>[2x]MGSSHHHHHHSQDPGDENLYFQSMSDADRIAALLKDRAADPVTKFSPSPYETGQFLRISERADVGTPQIDYLLATQRPDGLWGSVGFELVPTLGAVAGLSSRPEYADRAGVTDAVARACEKLWELALGEGGLPRLPDTVASEIIVPSLIDLLGEVLQRHRPAAGGKAGHEQEFPSPPGAKPELWRRLSDRIARGQAIPETAWHTLEAFHPLPEQFAATVTPAADGAVTCSPSSTAAWVSAVGTDAGASTRAYLDEAQSRYGGAIPMGSS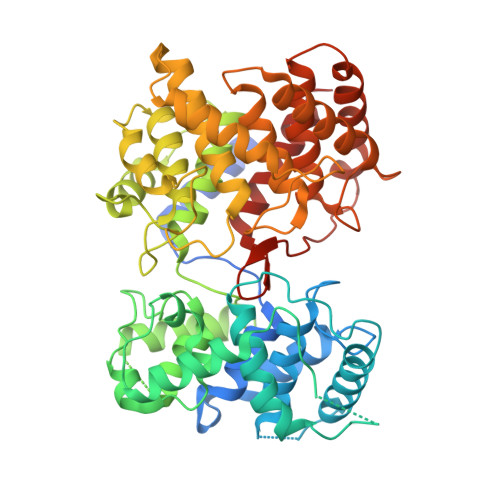MPYFEVLWVLNLVLKYFPDVPIPREIIEEIAAGFSESGIGGGPGLPPDGDDTAYANLAGDKLGAPTHPEILMKFWAEDHFVSYPGEQTPSETVNAHALEYLNHLRLRRGIAEYGAVEDACAEWVISQQTEDGCWYDKWNVSPYYSTAACVEALLDARKQDEPQLDSLRRAREWLLRHQTDSGGWGMAEPSPEETAYAVMALDLFASRGGKGAEECAAAISRAKEFFKDESRENPPLWMGKDLYTPFRIVEVTVMCGRAVVSRY> PISPIETVPVKLKPGMDGPKVKQWPLTEEKIKALVEICTEMEKEGKISKIGPENPYNTPVFAIKRKDSTKWRKLVDFRELNKRTQDFWEVQLGIPHPAGLKKKKSVTVLDVGDAYFSVPLDEDFRKYTAFTIPSINNETPGIRYQYNVLPQGWKGSPAIFQSSMTKILEPFKKQNPDIVIYQYMDDLYVGSDLEIGQHRTKIEELRQHLLRWGLTTPDKKHQKEPPFLWMGYELHPDKWTVQPIVLPEKDSWTVNDICKLVGKLNWASQIYPGIKVRQLSKLLRGTKALTEVIPLTEEAELELAENREILKEPVHGVYYDPSKDLIAEIQKQGQGQWTYQIYQEPFKNLKTGKYARMRGAHTNDVKQLTEAVQKITTESIVIWGKTPKFKLPIQKETWETWWTEY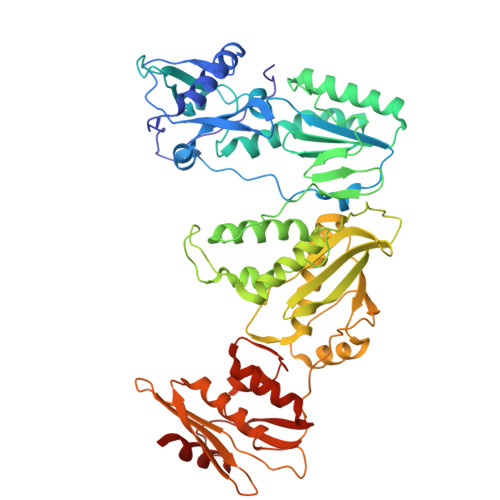WQATWIPEWEFVNTPPLVKLWYQLEKEPIVGAETFYVDGAANRETKLGKAGYVTNKGRQKVVPLTNTTNQKTELQAIYLALQDSGLEVNIVTDSQYALGIIQAQPDKSESELVNQIIEQLIKKEKVYLAWVPAHKGIGGNEQVDKLVSAGIRK> MIPGSFDYHRPKSIADAVALLTKLGEDA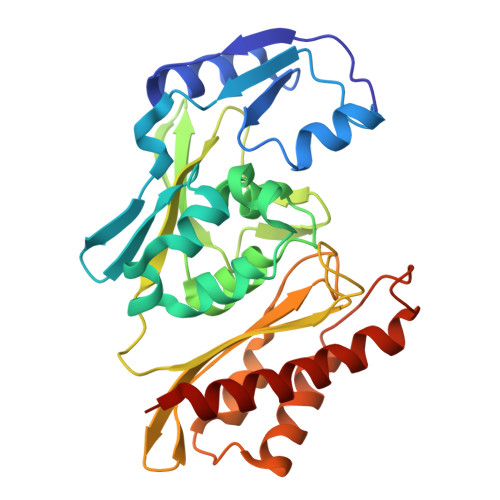RPLAGGHSLIPIMKTRLATPEHLVDLRDIGDLVGIREEGTDVVIGAMTTQHALIGSDFLAAKLPIIRETSLLIADPQIRYMGTIGGNAANGDPGNDMPALMQCLGAAYELTGPEGARIVAARDYYQGAYFTAIEPGELLTAIRIPVPPTGHGYAYEKLKRKIGDYATAAAAVVLTMSGGKCVTASIGLTNVANTPLWAEEAGKVLVGTALDKPALDKAVALAEAITAPASDGRGPAEYRTKMAGVMLRRAVERAKARAKN> MEESQSKQESNTRVAQHGSQQDVDPTFQTKRALEKERSKPRPRPLPRVQLQSLPGWSSTSKDVPLSQLIREMDHESRRCIHRSKKKLDRSEHISQGTIPEIYEKRKETISHTQSMEQKYLFQNFTKLLLLQKCCPGGSEKLVRESWHPCVPEEGGHMIEIQDLFDPNLDTEKKPQLVIIEGAAGIGKSTLARQVKRAWDEGQLYRDRFQHVFFFSCRELAQCKQLSLAELIAQGQEVPTAPTRQILSRPEKLLFILDGIDEPAWVLEDQNPELCVHWSQAQPVHTLLGSLLGKSILPEASLMLTARTTALQKLVPSLGQPHRVEVLGFSEFERKDYFYKYFAKERNTIIDFNLIGSIPVLLTLCEVPWVCWLLCTCLEKQMQQGEVLSLTSQTTTALCLKYLSLTIPGQHLSTQLRTLCS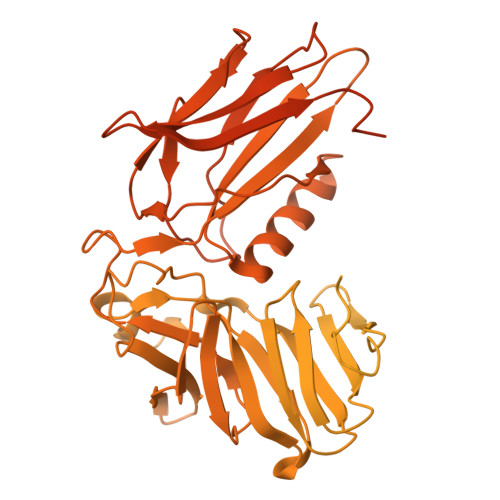LAAEGICQRRTLFSKSDLCKQGLAEDAIATFLKIGVLQRQPSSLSYSFAHLCLQEFFAAMSYILEDSEEAHGDMGNDRTVETLVERYGRQNLFEAPTVRFLLGLLNTREMREMENIFACKFPWETKLKLLQSIIGEPFCQPCHLGLFHCLYENQEEELLTETMLCFPLTASGPNHMEATVFQTNVKRLVIQTDMELMVVTFCITFSHVRSLRLKGKGQQEYKLTAPAMVLYRWTPISEASWKVLFSNLKCTRNLEELDLSGNPLSYSAVRSLCTALRQPGCRLKTLWLVDCGLTSRCCSFLASMLSAHSRLAELDLRLNDLGDNGVRQLCEGLRNPACNLSILRLDQASLSEQVITELRALETKNPKLFISSTWMSHMTMPTENTDGEESLTSSKQQQQQSGDKHMEPLGTDDDFWGPSGPVSTEVVDRERNLYRVRLPMAGSYHCPSTGLHFVVTRAVTIEIGFCAWSQFLHETPLQHSHMVAGPLFDIKAEHGAVTAVCLPHFVSLQEGKVDSSLFHVAHFQDHGMVLETPARVEPHFAVLENPSFSPMGVLLRMIPAVGHFIPITSITLIYYRLYLEDITFHLYLVPNDCTIRKAIDEEELKFQFVRINKPPPVDALYVGSRYIVSSSKEVEILPKELELCYRSPRESQLFSEIYVGNIGSGINLQLTDKKYMNLIWEALLKPGDLRPALPRMASAPKDAPALLHFVDQHREQLVARVTSVDPLLDKLHGLVLSEEDYETVRAEATNQDKMRKLFRGSRSWSWDCKDHFYQALKETHPHLIMDLLEKSGGVSVRL BROMO-DODECANOL | C12 H25 Br O | 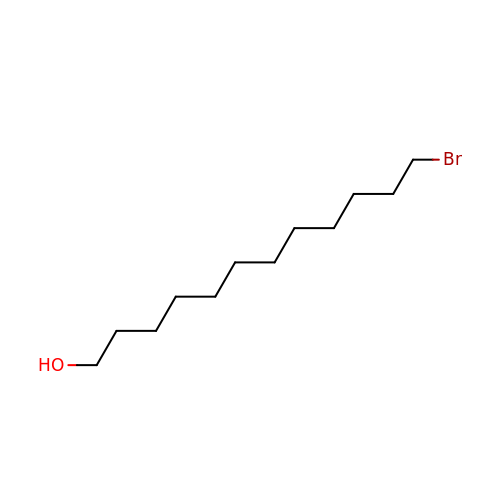ASIDMJNTHJYVQJ-UHFFFAOYSA-N> GTMTFQFRNPNFGGNP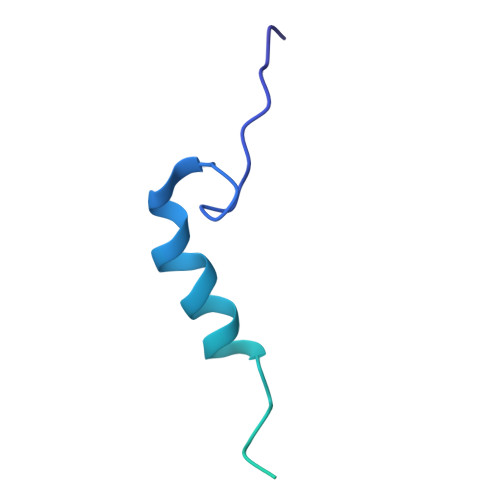NNGAFLLNSAQAQNSYKDPSYNDDFGIETPSALDNFTQAIQSQILGGLLSNINTGKPGRMVTNDYIVDIANRDGQLQLNVTDRKTGQTSTIQVSGLQNNSTDFHHHHHH7-{2-[2-(2,4-dioxo-3,4-dihydropyrimidin-1(2H)-yl)ethoxy]-4-fluorophenoxy}-5,8-dimethylnaphthalene-2-carbonitrile | C25 H20 F N3 O4 | 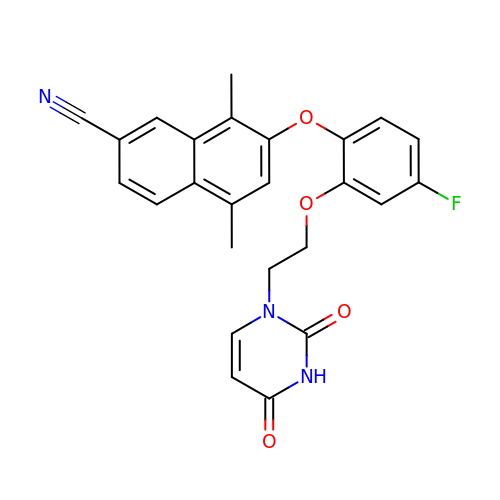JOZUOHBWIKONKE-UHFFFAOYSA-N(3R)-3-{[(BENZYLOXY)CARBONYL]AMINO}-2-OXO-4-PHENYLBUTANE-1-DIAZONIUM 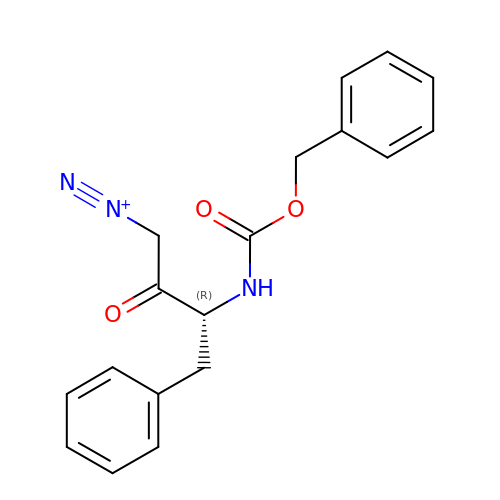| C18 H18 N3 O3 | VLIGBVLLNSWVMI-MRXNPFEDSA-O Pks13 is a multidomain enzyme that performs the final step in the synthesis of mycolic acids through the condensation of a long-chain fatty acid (C24–C26) and a very long-chain fatty acid (C56).12 The product is transferred from Pks13 to trehalose by the Pks13-TE domain. Pks13 fulfills a critical function for Mtb by performing a condensation reaction of a long-chain fatty acid and a very long-chain meromycolic acid to form a mycolic acid. Pks13-TE is a validated target for the development of antibiotics for Mtb. In previous work, we identified TAM16, a potent lead molecule for Pks13-TE. X-ray crystallography verified that compounds from all three different series were binding deep within the active site of Pks13-TE, displacing the side chain of Arg1563 with atoms within about 4 Å from the catalytic Ser1533 OG.

The DEL screen series 1 hit X20403 came from a library of over 2.8 billion compounds. X20403 showed potent activity with an IC50 of 57 nM in the Pks13-TE enzyme assay and 0.5 μM in the TAMRA binding assay. The cocrystal with X20403 solved at 2.0 Å resolution demonstrated a similar binding pose as X20404. Interestingly, the cyclopropyl group induced a shift of the α-helix formed by residues Lys1572-Lys1588, pulling the C-terminus of the helix closer to the inhibitor by 5.5 Å, as measured at the C-alpha of Phe1585. An additional H-bond was observed between the terminal methoxy O2 of the compound and ND2 of Asn1640. The side chains of Tyr1582 and Phe1585 are within VDW distance to C39 of the cyclopropyl group. Likely due to this gross change in the overall structure of the protein, crystals obtained for the X20403 complex packed differently, and the structure was solved in the P2221 space group, containing two protein molecules in the asymmetric unit, each bound to an inhibitor.

>IDGFVRTLRARPEAGGKVPVFVFHPAGGSTVVYEPLLGRLPADTPMYGFERVEGSIEERAQQYVPKLIEMQGDGPYVLVGWSLGGVLAYACAIGLRRLGKDVRFVGLIDAVRAGEEIPQTKEEIRKRWDRYAAFAEKTFNVTIPAIPYEQLEELDDEGQVRFVLDAVSQSGVQIPAGIIEHQRTSYLDNRAIDTAQIQPYDGHVTLYMADRYHDDAIMFEPRYAVRQPDGGWGEYVSDLEVVPIGGEHIQAIDEPIIAKVGEHMSRALGQIEADR[2x]>MSRVAPRDSAAQAASAVAESVRYQGRKASRQGSEQRRQAILDAAMRLIVRDGVRAVRHRAVAAEAQVPLSATTYYFKDIDDLITDTFALFVERNAEALSAFWSSVEGDLQEMAAVLADDPGARGSLVERIVELAVQYVQVQLTERREHLLAEQAFRQEALLNPRLRELADAHQRILSLGAVHFFQVLGSGQPEQDAKVLTSIILQ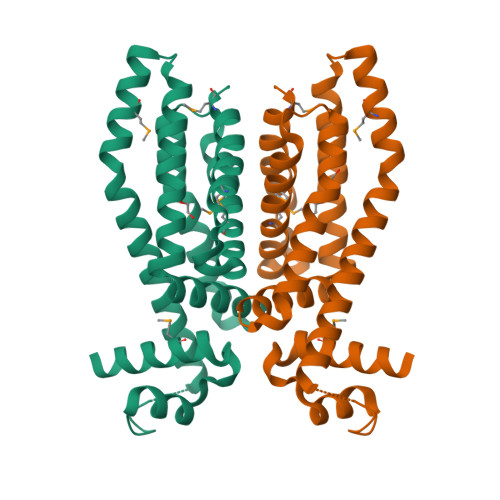MEYQGLVDGVEQLAVDEMRAILRRYLNLVMGL[3x]> ANKVIQLQKIFQSSTKPLWWRHPRSALY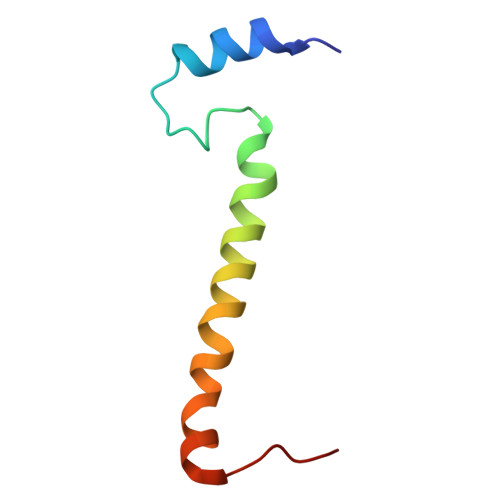LYPFYAIFAVAVVTPLLYIPNAIRGIKAKKA LINOLEIC ACID | C18 H32 O2 | 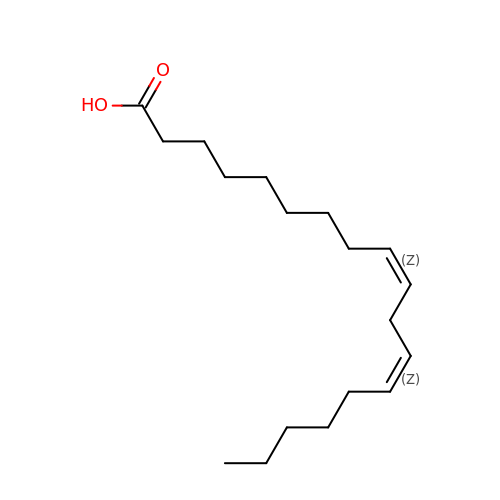OYHQOLUKZRVURQ-HZJYTTRNSA-N> MTMSRRNTDAITIHSILDWIEDNLESPLSLEKVSERSGYSKWHLQRMFKKETGHSLGQYIRSRKMTEIAQKLKESNEPILYLAERYGFESQQTLTRTFKNYF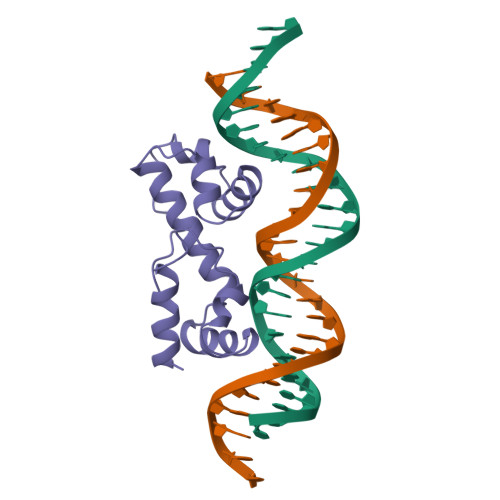DVPPHKYRMTNMQGESRFLHPLNHYNS>[2x]AKPCTVSTTNATVDLGDLYSFSLMSAGAASAWHDVALELTNCPVGTSRVTASFSGAADSTGYYKNQGT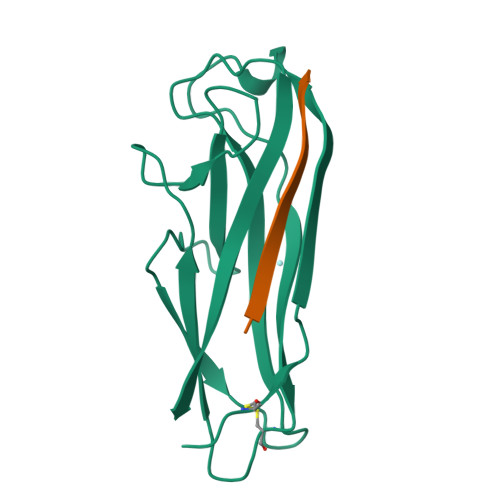AQNIQLELQDDSGNTLNTGATKTVQVDDSSQSAHFPLQVRALTVNGGATQGTIQAVISITYTYS;>[2x]ADSTITIRGYVRDNR> GPDSMASVTLSEAEK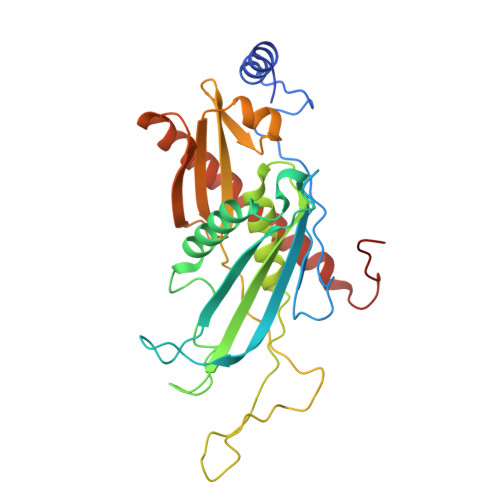VYIVHGVQEDLRVDGRGCEDYRCVEVETDVVSNTSGSARVKLGHTDILVGVKAEMGTPKLEKPNEGYLEFFVDCSASATPEFEGRGGDDLGTEIANTLYRIFNNKSSVDLKTLCISPREHCWVLYVDVLLLECGGNLFDAISIAVKAALFNTRIPRVRVLEDEEGSKDIELSDDPYDCIRLSVENVPCIVTLCKIGYRHVVDATLQEEACSLASLLVSVTSKGVVTCMRKVGKGSLDPESIFEMMETGKRVGKVLHASLQSVVHKEESLGPKRQKVGFLG>SNAIGGAVKLSISYRNGTLFIMVMHIKDLVTEDGADPNPYVKTYLLPDNHKTSKRKTKISRKTRNPTFNEMLVYSGYSKETLRQRELQLSVLSAESLRENFFLGGVTLPLKDFNLSKETVKW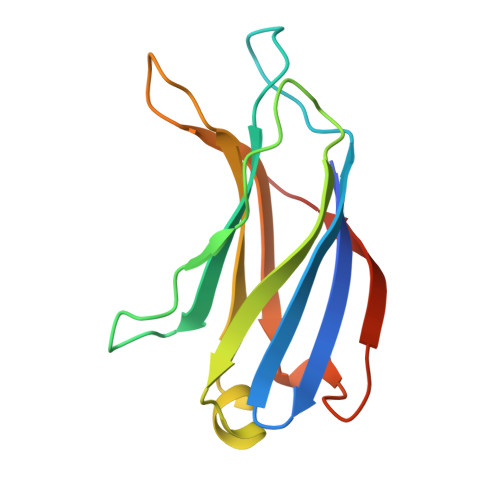YQLTAATYL[2x]>NISVPSSPPGGERVGILGAGIGGLYSALILQSLDVPFEIIEASNRVGGRLFTHKFPNGGKYDYYDVGAMRYPLPKSDDKGNYQPGVMQRVGQLFTYLGMHKQLIPYYFKSNKSPGFQYFNGVRARIGEGSSFDAPALGINSSLIDIGVTKIVNDAVGPFAQALFDDLQKHTTTGWDDMMKNDAYSTRSYFSFKYLPSPSFGLPSEHFSTRVINWLETFDKSTGWYDRGLTETVLEAIAFGEVGDGEVDWRCIDGGSHVLPDTIAAFLHKKGGNAFVMNASVTAIGLENPNKEDSPMVVV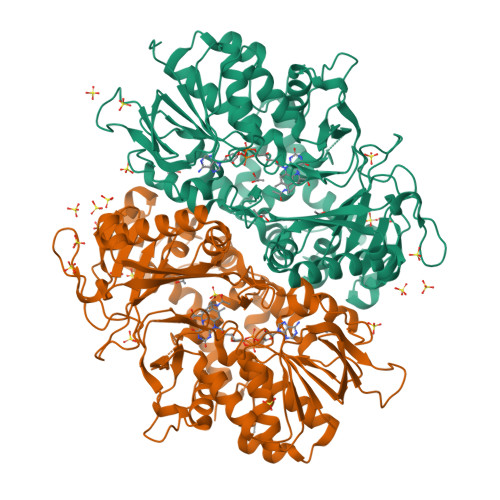AGGQKRKYSHVISTLPLPVLRTVDLKNSKLDIVQSNALRKLQYGPSIKIGILFKEPWWTTGQDKNGEKFDLVGGQSYTDLPIRTVVYPSYGVNTNAPSNTLIASYCWTNDAERMGSLIGTGAATYEEQLEHLVLSNLAAVHNTDYQYLKDRLVDVHSWDWNHNPLTMGAFAFFGPGDFQDLYTSLNRPAANGKLHFAGEALSVRHAWVVGALDSAWRAVYNYLYVTDPAKLPKFFELWGKNAEWFEQPGDGKEPNSDNSLLEK[4x]RIP2 has a C-terminal CARD domain presumably perceiving the upstream activation signal, and an N-terminal kinase domain that could dimerize and phosphorylate other downstream factors, including TAK1 and NF-κB. After depletion of the intrinsic RIP2 in HEK293T cells, both NOD1/2 full-length and NOD1/2 CARD domains failed to activate NF-κB, which demonstrates that RIP2 is the predominant downstream signaling adapter for NOD1/2. In this study, we demonstrated that the innate immune adapter RIP2 forms a helical oligomeric structure upon activation. Loss-of-function mutations in NOD1/2 and RIP2 are associated with autoimmune diseases, such as Crohn’s disease and lupus.

Second, we reconstituted homogeneous RIP2–CARD filaments and determined the 4.1-Å resolution cryo-EM structure of the active complex. We then constructed the atomic model of RIP2–CARD filament and validated it using pairwise charge-reversal mutagenesis. These findings provided a direct view of how RIP2–CARD is organized in a C1 left-handed helical filament upon activation. A 13 amino acid tag was added to the N-terminal of residue 432 of RIP2–CARD and the last 11 amino acids at the C-terminal end of RIP2–CARD were removed to stabilize the core RIP2–CARD filament and prevent filament bundling on the EM grid. As a typical Type I interface, residues from helix 1 and 4 (orange, Type Ia, R444, E445, and D492) interact with charged side chains from helix 2 and 3 (red, Type Ib, Q458, D461, Y474, and K471). In Type II interactions, residues at the turns between helix 2/3 and helix 4/5 (orange, Type IIa, D495, Q497, E472, and D467) mainly interact with residues located within the turn between helix 1/2 (green, Type IIb, N449, T452, and K513). Type III (orange and blue) interface was relatively weak and it was stabilized by interactions between residues from helix 2 (orange, Type IIIa, T479, E475, K471, and E472) and coiled turn between helix 3/4 (blue, Type IIIb, R483, T482, T484, and R488). Overall, the stability of the RIP2–CARD filament was maintained by a collection of weak charged interactions involving almost all surfaces of RIP2–CARD. Cellular activities were completely abolished when we disrupted the native interaction pairs E445–Q458 and N449–D495. When the interactions at these sites were rescued by introducing reversely charged interactions pairs, E445R–Q458E double mutant regained its activity and was six times more active than any of the single mutants.

>TNSAGIAQQWIQSKREDIVNQMTEACLNQSLDALLSRDLIMKEDYELVSTKPTRTSKVRQLLDTTDIQGEEFAKVIVQKLKDNKQMGLQPYPEILVVSRSPSLNLLQNKSM[12x]>[3x]MATPASGALLQQMNLASQSLNYELSFISINKQGVESLRYRHARLDNRPLAQLLQMDGPRREVVQRGNEISYFEPGLEPFTLNGDYIVDSLPSLIYTDFKRLSPYYDFISVGRTRIADRLCEVIRVVARDGTRYSYIVWMDTESKLPMRVDLLDRDGETLEQFRVIAFNVNQDISSSMQ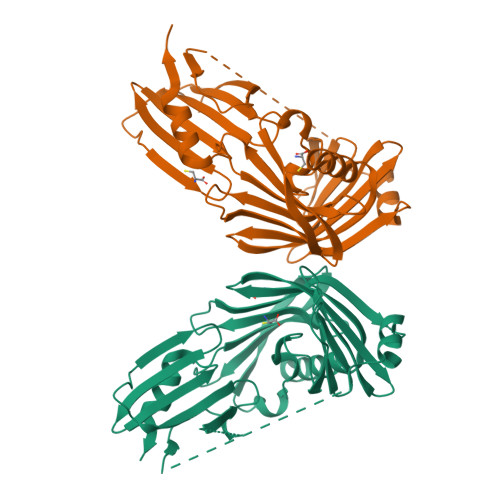TLAKANLPPLLSVPVGEKAKFSWTPTWLPQGFSEVSSSRRPLPTMDNMPIESRLYSDGLFSFSVNVNRATPSSTDQMLRTGRRTVSTSVRDNAEITIVGELPPQTAKRIAENIKFGAAQHHHHHH1,4-anhydro-D-erythro-pent-1-enitol | C5 H8 O4 | 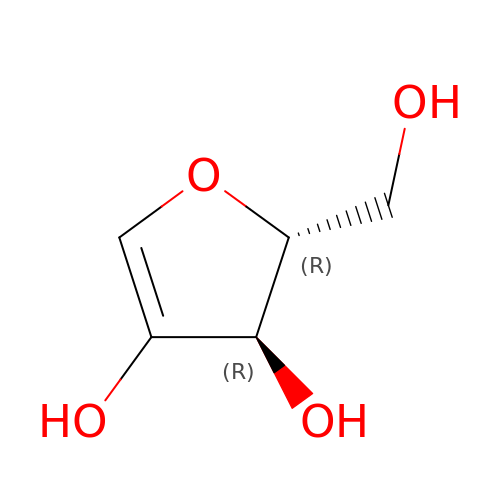WGCMRWDTTZWXPL-UHNVWZDZSA-N>[3x]MAMKRLLVTGAAGQLGRVMRERLAPMAEILRLADLSPLDPAGPNEECVQCDLADANAVNAMVAGCDGIVHLGGISVEKPFEQILQGNIIGLYNLYEAARAHGQPRIVFASSNHTIGYYPQTERLGPDVPARPDGLYGVSKCFGENLARMYFDKFGQETALVRIGSCTPEPNNYRMLSTWFSHDDFVSLIEAVFRAPVLGCPVVWGASANDAG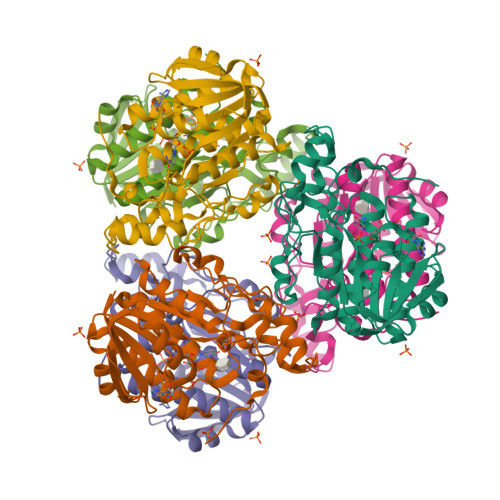WWDNSHLGFLGWKPKDNAEAFRRHITETTPPPDPNDALVRFQGGTFVDNPIFKQS>TELTKCKVSHAIKDIDGYQGISLLEWACVLFHTSGYDTQAVVNDNGSTEYGLFQ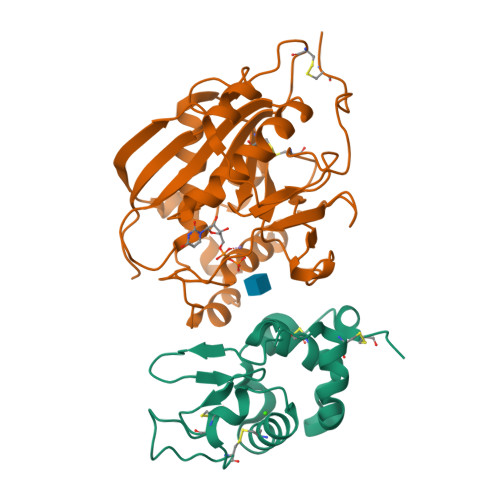ISDRFWCKSSEFPESENICGISCDKLLDDELDDDIACAKKILAIKGIDYWKAYKPMCSEKLEQWRCEKP[2x];>[2x]ASMTGGQQMGRGSSLTACPEESPLLVGPMLIEFNIPVDLKLVEQQNPKVKLGGRYTPMDCISPHKVAIIIPFRNRQEHLKYWLYYLHPILQRQQLDYGIYVINQAGESMFNRAKLLNVGFKEALKDYDYNCFVFSDVDLIPMNDHNTYRCFSQPRHISVAMDKFGFSLPYVQYFGGVSALSKQQFLSINGFPNNYWGAGGEDDDIYNRLAFRGMSVSRPNAVIGKTRMIRHSRDKKNEPNPQRFDRIAHTKETMLSDGLNSLTYMVLEVQRYPLYTKITVDIGTPS>MNGAIKVGAWGGNGGSAFDMGPAYRIISVKIFSGDVVDGVDVTFTYYGKTETRHYGGSGGTPHEIVLQEGEYLVGMAGEVANYHGAVVLGKLGFSTNKKAYGPFGNTGGTPFSL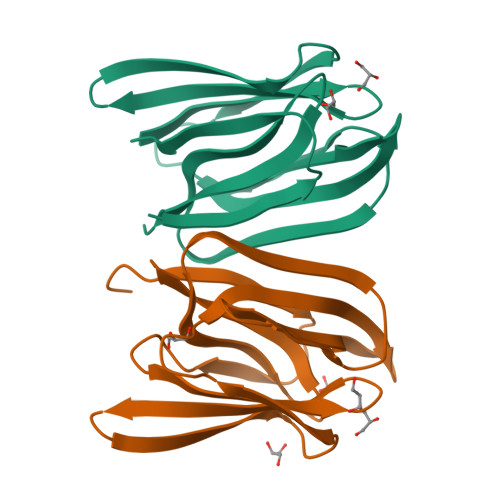PIAAGKISGFFGRGGKFLDAIGVYLEPLEHHHHHH[4x]>SNAFHQISSRIQKSIDVDEVLRLCAEGLHDVLGYERVNILMADTARTSLSFVAAVGTADFNPAGVVLPLDQRGGVITKCFTDRQVYMIDDVSAYPTDFRLQSPYDAIRALRSKSFVICPIVVKGEAIGVFAVD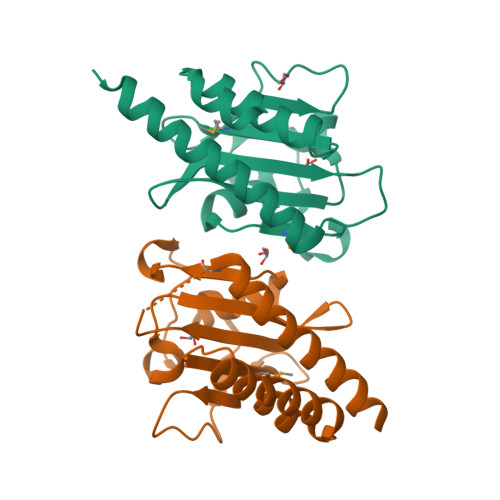NRSSRRSLNDTDVDTIKLFADQASSAIVRINLLKAI[2x]>MPVDKNLRDLEPGIHTDLEGRLTYGGYLRLDQLLSAQQPLSEPAHHDEMLFIIQSQTSELWLKLLAHELRAAIVHLQRDEVWQCRKVLARSKQVLRQLTEQWSVLETLTPSEYMGFRDVLGPSSGFQSLQYRYIEFLLGNKNPQMLQVFAYDPAGQARLREVLEAPSLYEEFLRYLARFGHAIPQQYQARDWTAAHVADDTLRPVFERIYENTDRYWREYSLCEDLVDVETQFQLWRFRHMRTVMRVIGF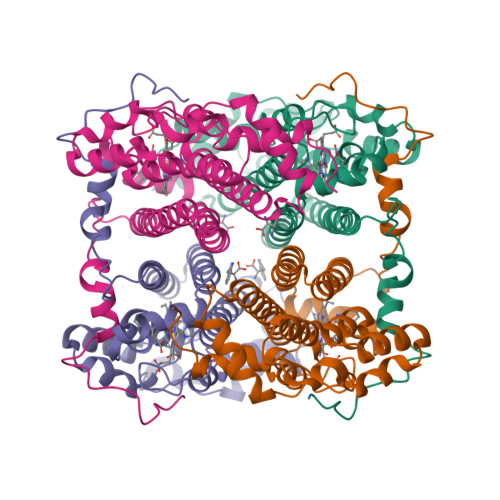KRGTGGSSGVGFLQQALALTFFPELFDVRTSVGVDNRPPQGSADAGKR[8x]>[2x]MHRSPLAWLRLLLAAVLGAFLLGGPLHAAETAATRSPAWAQAVDPSINLYRMS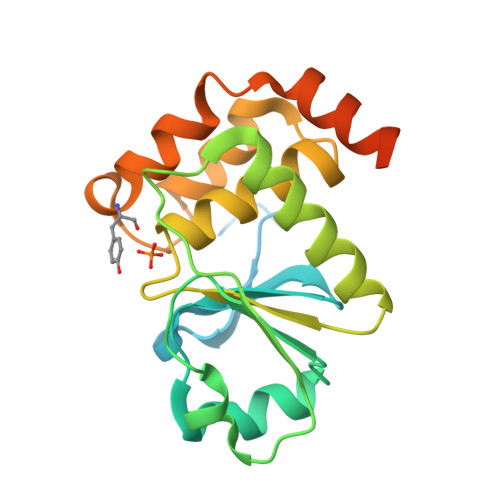PTLYRSALPNAQSVALLQRLQVKTVVSFIKDDDRAWLGQAPVRVLSLPTHADRVDDAEVLSVLRQLQAAEREGPVLMHSKHGNNRTGLFAAMYRIVVQGWDKQAALEEMQHGGFGDEDDMRDASAYVRGADVDGLRLAMANGECSPSRFAVCHVREWMAQALDRP>GMARCERLRGAALRDVLGQAQGVLFDCDGVLWNGERIVPGAPELLQRLARAGKNTLFVSNNSRRARPELALRFARLGFAGLRAEQLFSSALCAARLLRQRLSGPPDASGAVFVLGGEGLRAELRAAGLRLAGDPGEDPRVRAVLVGYDEQFSFSRLTEACAHLRDPDCLLVATDRDPWHPLSDGSRTPGTGSLAAAVETASGRQALVVGKPSPYMFQCITEDFSVDPARTLMVGDRLETDILFGHRCGMTTVLTLTGVSSLEEAQAYLTAGQRDLVPHYYVESIADLMEGLEE[2x]

Pyridoxal 5’-phosphate phosphatase (PDXP), an enzyme that controls levels of pyridoxal 5’-phosphate (PLP), the co-enzymatically active form of vitamin B6, may represent an alternative therapeutic entry point into vitamin B6-associated pathologies. PDXP is a member of the large family of haloacid dehalogenase (HAD)-type hydrolases. HAD phosphatases are Mg2+-dependent phospho-aspartate transferases that consist of a Rossman-like catalytic core linked to a cap domain. 7,8-DHF binds and reversibly inhibits PDXP with low micromolar affinity and sub-micromolar potency.

7,8-DHF-bound murine PDXP co-crystallized with phosphate in the cubic space group I23, with protomer A containing the inhibitor and protomer B representing an inhibitor-free state. 7,8-DHF was observed to only bind to one subunit (the A-chain) of murine PDXP with well-defined density and full occupancy since its average B-factor of 45.8 Å2 closely matches the B-factors of the surrounding atoms. Binding to the other subunit (B-protomer) is prevented by a salt bridge between Arg62 and Asp14 of a symmetry-related A-protomer in the crystal. To allow binding of the inhibitor, the side chain of Arg62 needs to adopt a completely extended conformation, which is prevented by the salt bridge. However, preventing mPDXP salt bridge formation by mutating Asp14 to Ala did not alter the efficacy of 7,8-DHF inhibition (see also Figure 3d for the characterization of the PDXP-Arg62Ala variant). Due to the limited solubility of 7,8-DHF, we were unable to address the stoichiometry of 7,8-DHF binding to the PDXP dimer with isothermal calorimetry. It is conceivable that the mPDXP crystal packing is very stable (indeed, 7,8-DHF-bound mPDXP crystallized in the same cubic space group as apo-mPDXP, see Kestler et al., 2014, including the aforementioned salt bridge between Arg62 of the B-subunit and Asp14 of a symmetry-related molecule), and that the free energy generated by the formation of the crystal lattice is higher than the free energy generated upon inhibitor binding. The Cα atom-based alignment of the structures representing murine apo-PDXP and murine 7,8-DHF-bound PDXP resulted in root mean square (RMS) deviations in the range of 0.43–0.71 Å. The inhibitor localization in the presence of phosphate was identical in human and murine PDXP. Inhibitor binding in the presence of phosphate is identical in human and murine PDXP and appears to be primarily stabilized by two hydrogen bonds, as well as polar and non-polar interactions.>[2x]GMGILSGNPQDEPLHYGEVFSTWTYLSTNNGLINGYRSFINHT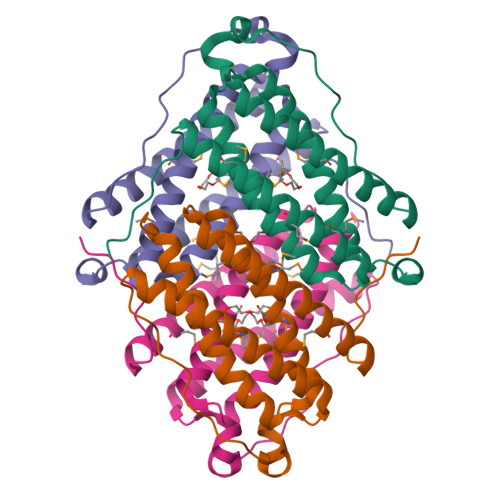GDEDLKNLIDEAIQAMQDENHQLEELLRSNGVGLPPAPPDRPAARLDDIPVGARFNDPEISATISMDVAKGLVTCSQIIGQSIREDVALMFSQFHMAKVQFGGKMLKLNKNKGWLIPPPLHSDRPIKE>[10x]MLVSVYLALLVACVGQAHSQANLMRLKSDLFNRSPMYPGPTKDDPLTVTLGFTLQDIVKVDSSTNEVDLVYWERQRWKLNSLMWDPNEYGNITDFRTS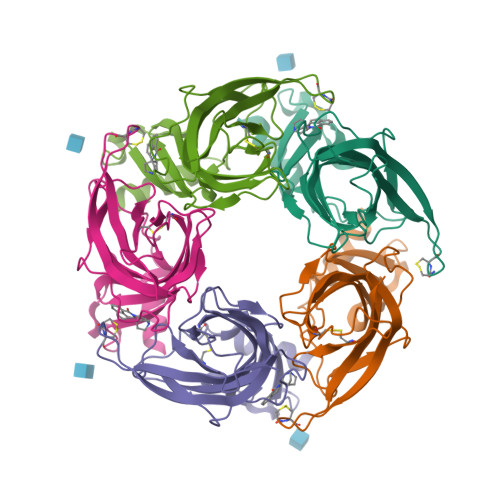AADIWTPDITAYSSTRPVQVLSPQIAVVTHDGSVMFIPAQRLSFMCDPTGVDSEEGVTCAVKFGSWVYSGFEIDLKTDTDQVDLSSYYASSKYEILSATQTRQVQHYSCCPEPYIDVNLVVKFRERRAGNGFFRNLFDHHHHHH Inositol pyrophosphates (PP−IPs) are densely phosphorylated messenger molecules involved in numerous biological processes. To investigate the function and regulation by PP−IPs in biological contexts, metabolically stable analogs have been developed. Co‐crystallization with the proteins DIPP1 and PPIP5K2 enabled us to scrutinize similarities and disparities of all analogs, as compared to 5PP−IP5. The DIPP1 phosphatase has a flexible ligand binding domain whereas the PPIP5K kinase domain displays higher ligand specificity.

To address this issue, the Potter group recently developed an α‐phosphono‐α,α‐difluoroacetamide analog, 5PCF2Am−IP5. In this analog, the pyrophosphate mimicking group is bound to the inositol ring via an amide bond, which is less prone to hydrolysis than esters. The DIPP1/5PCF2P−IP5 structure included the four Mg2+ atoms we identified in a previous study with the natural substrate 5PP−IP5. It is interesting that, relative to 5PP−IP5, the 5PCF2P−IP5 is flipped approximately 180° across the C2−C5 axis into a non‐productive orientation (i. e., it does not mimic the catalytically‐productive positioning of the 5PP−IP5 β‐phosphate). An almost identical positioning was observed for 5PCF2Am−IP5 in DIPP1 crystals. These non‐productive ligand presentations also resemble those of 5PCF2Am−IP5 in a crystal complex with the S. cerevisiae Ddp1. Perhaps for DIPP1 this particular binding mode is the result of a biologically irrelevant stabilization, promoted by the fortuitous positioning of the fluorine atoms that facilitates polar interactions with R89. Although the fluorinated analogs have protonation states that are closer to the natural molecule at physiological pH, the introduction of the fluorine atoms leads to the formation of a polar interaction with a nearby arginine residue, favouring the flipped orientation. Given the high density of positively charged residues in PP−IP binding sites, it seems likely that such polar interactions between fluorine and neighboring lysine or arginine side chains can contribute to the binding orientation and binding strength of the fluorinated analogs.

> MMKLKSNQTRTYDGDGYKKRAACLCFRSESEEEVLLVSSSRHPDRWIVPGGGMEPEEEPSVAAVREVCEEAGVKGTLGRLVGIFENQERKHRTYVYVLIVTEVLEDWEDSVNIGRKREWFKIEDAIKVLQYHKPVQASYFETLRQGYSANNGTPVVATTYSVSAQSSMSGIR(4~{S},6~{S})-4-[2,4-bis(fluoranyl)phenyl]-4-methyl-6-pyrimidin-5-yl-5,6-dihydro-1,3-thiazin-2-amine 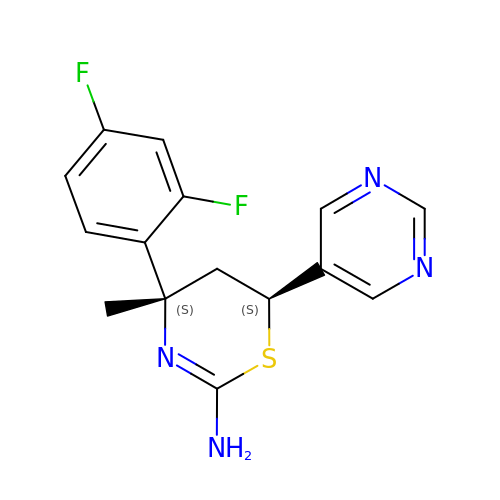| C15 H14 F2 N4 S | AHFBBIPUKVCJEP-ZFWWWQNUSA-N>[2x]MKKVKLIGTLDYGKYRYPKNHPLKIPRVSLLLRFKDAMNLIDEKELIKSRPATKEELLLFHTEDYINTLMEAERSQSVPKGAREKYNIGGYENPVSYAMFTGSSLATGSTVQAIEEFLKGNVAFNPAGGMHHAFKSRANGFCYINNPAVGIEYLRKKGFKRILYIDLDAHHCDGVQEAFYDTDQVFVLSLHQSPEYAFPFEKGFLEEIGEGKGKGYNLNIPLP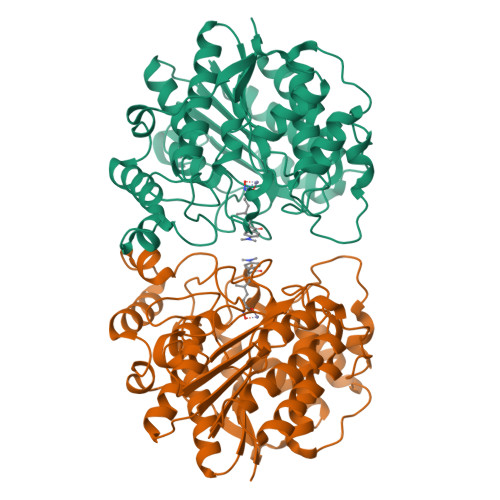KGLNDNEFLFALEKSLEIVKEVFEPEVYLLQLGTDPLLEDYLSKFNLSNVAFLKAFNIVREVFGEGVYLGGGGYHPYALARAWTLIWCELSGREVPEKLNNKAKELLKSIDFEEFDDEVDRSYMLETLKDPWRGGEVRKEVKDTLEKAKASS> MIKIGAHMPISKGFDRVPQDTVNIGGNSFQIFPHNARSWSAKLPSDEAATKFKREMKKHGIDWENAFCHSGYLINLASPKDDIWQKSVELLKKEVEICRKLGIRYLNIHPGSHLGTGEEEGIDRIVRGLNEVLNNTEGVVILLENVSQ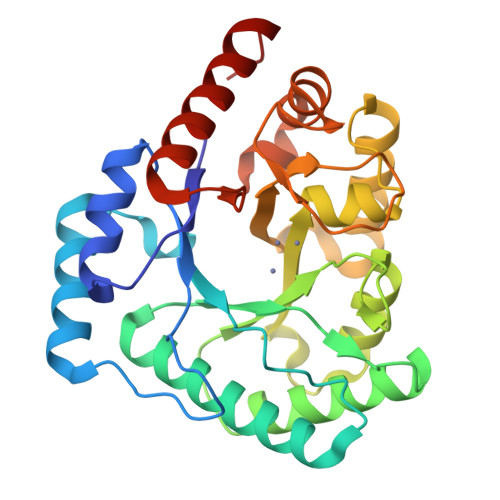KGGNIGYKLEQLKKIRDLVDQRDRVAITYDTCHGFDSGYDITKKEGVEALLNEIESLFGLERLKMIHLNDSKYPLGAAKDRHERIGSGFIGEEGFAVFFSFKEIQEVPWILETPGGNEEHAEDIKKVFEIIEKFGIEVD>[6x]MGSSHHHHHHSQDPSDQYPQTGTYPDVQTPYQIIKVDGSEKNGQHKALNPNPYERVIPEGTLSKRIYQVNNLDDNQYGIELTVSGKTVYEQKDMADLTEKKSIENGTITDPMGELIDLQLGTDGRFDPADYTLTANDGSRLENGQAVGGPQNDGGLLKNAKVLYDTTEKRIRVTGLYLGTDEKVTLTYNVRLNDEFVSNKFYDTNGRTTLHPKEVEQNTVRDFPIPKIRDVR

RrgA is the structural pilin positioned at the tip of S. pneumoniae pilus-1 and contains four unusual elongated domains. RrgA harbors two intramolecular isopeptide bonds, one located in the D2 domain, and the second in D4. The D2 domain is formed by the association of 2 “halves” encoded by sequences flanking the D3 domain. The distinct N-(residues 144–220) and C-terminal (residues 593–722) sub-domains, hereafter referred as Jo and In, respectively, clasp into an 11-β stranded sandwich locked by an isopeptide bond between the side chains of Lys191 in Jo and Asn695 in In.

We provide evidence that two engineered protein fragments from RrgA retain their ability to associate covalently in vivo and in vitro although being isolated from the parent protein. Altogether, these data show that Jo and In sub-domains retain their ability to form a stable complex although isolated from the parent RrgA protein. The amide bond formation between the Lys and the Asn side chains is dependent on Asp6008. The covalent complex His-Jo-His-In was formed only when both WT forms of Jo and In were mixed, while each point mutation totally impaired the complex assembly. The reaction was efficient at pH 8 and pH 7 since 100% of the complex was reconstituted after 1 h, the formation of the complex was slightly reduced to 90% at pH 6 and largely inefficient at pH 5 since only 18% of the complex could be detected. This pH dependency suggests that a residue, likely Asp600, with a pKa value between 5 and 6 might need to be deprotonated to participate in the reaction mechanism. The structure of the complex shows that the Jo and In moieties grasp into an 11-β-stranded sandwich. The two partners are locked together by the isopeptide bond formed by the fusion of the side chains of Lys191 and Asn695 in proximity to Asp600. The structure of the complex is indistinguishable from that of the RrgA D2 domain (rms of 0.61 Å), indicating that the fold adopted by the Jo and In partners produced individually, although possibly different from that acquired in the context of the full RrgA sequence, still remains compatible with the complex formation. Parental RrgA and Jo-In complex structures were superimposed and neither significant differences nor flexibility were detected despite slight variations observed in a few loops (depicted in Fig. 3e by arrows). The purified product, His-Jo-GSTPGSV-In, folds into a circular single polypeptide chain containing the covalent isopeptide bond as confirmed by ESI-MS.> GAMSVPAIAPRRKRLADGLSVTQKVFVRSRNGGATKIVREHYLRSDIPCLSRSCTKCPQIVVPDAQNELPKFILSDSPLELSAPIGKHYVVLDTNVVLQAIDLLENPNCFFDVIVPQIVLDEVRNKSYPVYTRLRTLCRDSDDHKRFIVFHNEFSEHTFVERLPNETINDRNNRAIRKTCQWYSEHLKPYDINVVLVTNDRLNREAATKEVESNII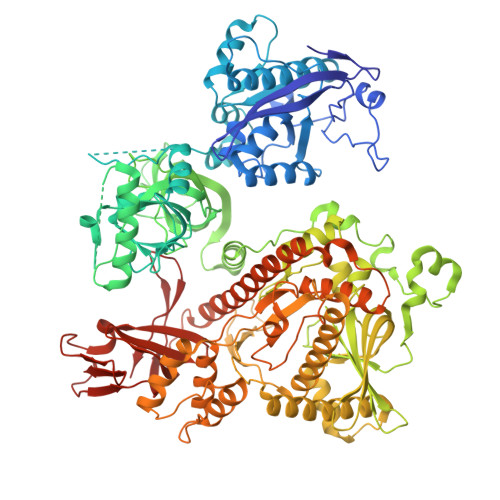TKSLVQYIELLPNADDIRDSIPQMDSFDKDLERDTFSDFTFPEYYSTARVMGGLKNGVLYQGNIQISEYNFLEGSVSLPRFSKPVLIVGQKNLNRAFNGDQVIVELLPQSEWKAPSSIVLDSEHFDVNDNPDIEAGDDDDNNESSSNTTVISDKQRRLLAKDAMIAQRSKKIQPTAKVVYIQRRSWRQYVGQLAPSSVDPQSSSTQNVFVILMDKCLPKVRIRTRRAAELLDKRIVISIDSWPTTHKYPLGHFVRDLGTIESAQAETEALLLEHDVEYRPFSKKVLECLPAEGHDWKAPTKLDDPEAVSKDPLLTKRKDLRDKLICSIDPPGCVDINDALHAKKLPNGNWEVGVHIADVTHFVKPGTALDAEGAARGTSVYLVDKRIDMLPMLLGTDLCSLKPYVDRFAFSVIWELDDSANIVNVNFMKSVIRSREAFSYEQAQLRIDDKTQNDELTMGMRALLKLSVKLKQKRLEAGALNLASPEVKVHMDSETSDPNEVEIKKLLATNSLVEEFMLLANISVARKIYDAFPQTAMLRRHAAPPSTNFEILNEMLNTRKNMSISLESSKALADSLDRCVDPEDPYFNTLVRIMSTRCMMAAQYFYSGAYSYPDFRHYGLAVDIYTHFTSPIRRYCDVVAHRQLAGAIGYEPLSLTHRDKNKMDMICRNINRKHRNAQFAGRASIEYYVGQVMRNNESTETGYVIKVFNNGIVVLVPKFGVEGLIRLDNLTEDPNSAAFDEVEYKLTFVPTNSDKPRDVYVFDKVEVQVRSVMDPITSKRKAELLLK>AMMEIDELTALGGLLHDIGKPVQRAGLYSGDHSTQGARFLRDLAENTGRAEYELLSLFSEFHHKGHMKNDELMIRRIKELSPERFGLTMEDVLNALWIVYEADNLASGEREEGQPQASRPLYSVFNPGKAYPWAELDFEKELPVPGDVFSIRSQDYRELVKRLWEELSKAKLRSDRLLPVLEKYLTFVSSVTSEGNIISLYDHMRMTSAIALAMLRAGCTAEDVRSGRCRKEKRFLLIEGDFSGIQDFIYRVSGKGTLKYLRARSAYLELIGWDVVLEILSRLGLTRANVVFNAGGHFMIIAQNTPDAVKELEEIRAKAVEWLYREFESDLYLAIEWEPVSGREFGREGGKNLFAEARKRLKHKLTVRKLKRFGEIKGLFEHGHTERLAECPVCGRELPEGKLEPSASDPETKVCPTCNRLVSLGGNLPKLLGFGRTAKNDAGVLVEGPFSGFVPYLQGGRPVGEQILVKNTLNPGEIPESAQFVPYFVADYFKKDPKGGVATFEELSMASTGTRRLGVMKGDVDRLGEFFSSMDSPSKLATASRFMDYFFKGYIGAIIEGKFGYIIGDVPSLRDWPEEPDIVVVYAGGDDFFIVGAWDQIFELAFRVRRAFNAYTGGKLTLSVGLGYFDERTPIYRMADVVSERLDTAK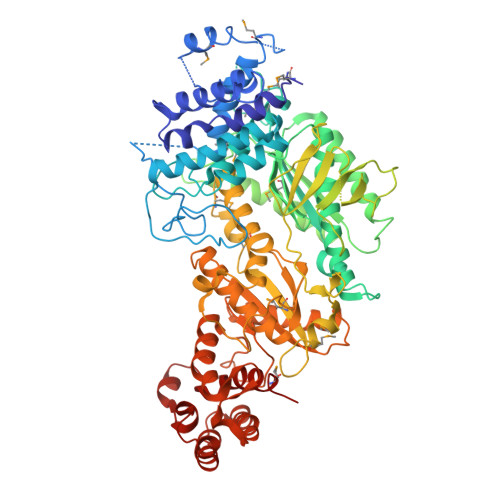DEGRNRVFVVGRSRPLDGKHKLSYEWNHYEELWRTYAPRIYAGNGRLKGKLESKKGLLWKLLEIRELYVRDPNDVRWAYLTAYLLGRHGLSDLFPELVGIDTKAVERKEPQPVYWVDGVLKIVLMAVRR[4x]> MHHHHHHSMGKRNKPGKATGKGKPVNNKWLNNAGKDLGSPVPDRIANKLRDKEFKSFDDFRKKFWEEVSKDPELSKQFSRNNNDRMKVGKAPKTRTQDVSGKRTS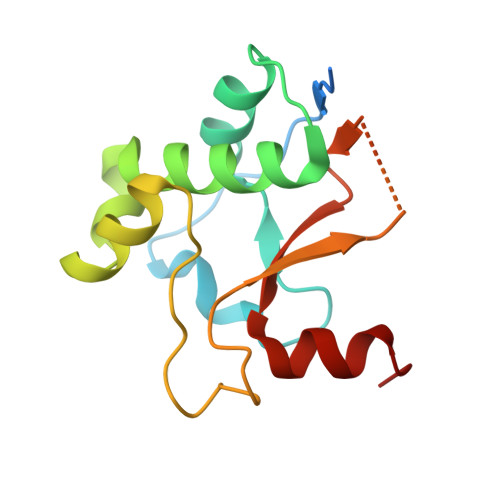FELHAEKPISQNGGVYDMDNISVVTPKRHIDIHRGK>MAQQTPLYEQHTLCGARMVDFHGWMMPLHYGSQIDEHHAVRTDA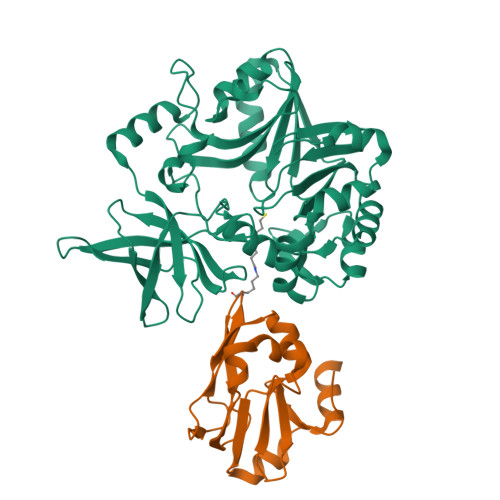GMFDVSHMTIVDLRGSRTREFLRYLLANDVAKLTKSGKALYSGMLNASGGVIDNLIVYYFTEDFFRLVVNSATREKDLSWITQHAEPFGIEITVRDDLSMIAVQGPNAQAKAATLFNDAQRQAVEGMKPFFGVQAGDLFIATTGYTGEAGYEIALPNEKAADFWRALVEAGVKPCGLGARDTLRLEAGMNLYGQEMDETISPLAANMGWTIAWEPADRDFIGREALEVQREHGTEKLVGLVMTEKGVLRNELPVRFTDAQGNQHEGIITSGTFSPTLGYSIALARVPEGIGETAIVQIRNREMPVKVTKPVFVRNGKAVA[4x];>MSNVPAELKYSKEHEWLRKEADGTYTVGITEHAQELLGDMVFVDLPEVGATVSAGDDCAVAESVKAASDIYAPVSGEIVAVNDALSDSPELVNSEPYAGGWIFKIKASDESELESLLDATAYEALLEDE[2x]> GSHMSPKIVDAGTATVPHTMSTMKTADNRPASVYLKKDKPTLIKFWASWCPLCLSELGQAEKWAQDAKFSSANLITVASPGFLHEKKDG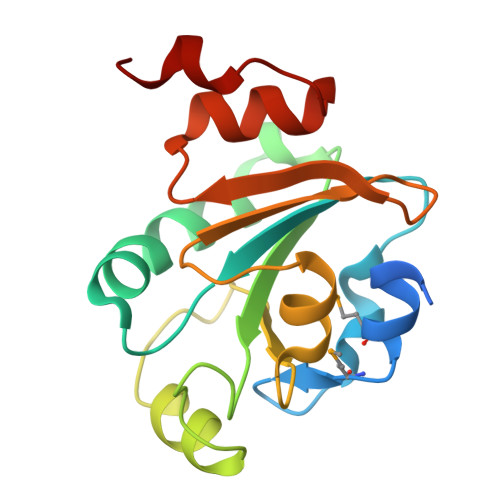EFQKWYAGLNYPKLPVVTDNGGTIAQNLNISVYPSWALIGKDGDVQRIVKGSINEAQALALIRNPNADLGSLKHS> KEVCYEQIGCFSDAEPWAGTAIRPLKVLPWSPERIGTRFLLYTNKNPNNFQTLLPSDPSTIGASNFQTDKKTRFIIHGFIDKGEENWLLDMCKNMFKVEEVNCICVDWKKGSQTSYTQAANNVRVVGAQVAQMLSMLSANYSYSPSQVQLIGHSLGAHVAGEAGSRTPGLGRITGLDPVEASFQGTPEEVRLDPTDADFVDVIHTDAAPLIPFLGFGTSQQMGHLDFFPNGGEEMPGCKKNALSQIVDLDGIWEGTRDFVACNHL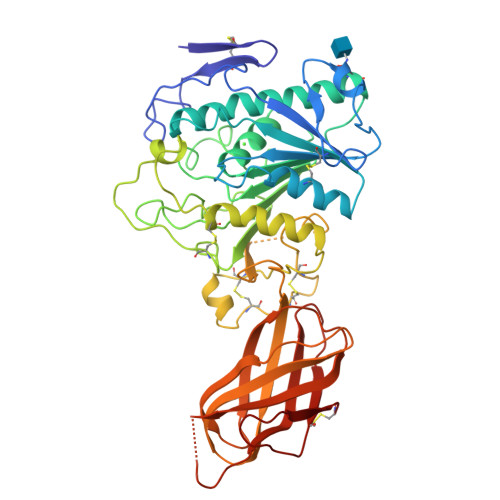RSYKYYSESILNPDGFASYPCASYRAFESNKCFPCPDQGCPQMGHYADKFAVKTSDETQKYFLNTGDSSNFARWRYGVSITLSGKRATGQAKVALFGSKGNTHQFNIFKGILKPGSTHSNEFDAKLDVGTIEKVKFLWNNNVVNPTFPKVGAAKITVQKGEEKTVHSFCSESTVREDVLLTLTPC>MRINHNIAALNTLNRLPSNNSASQKNMEKLSSGLRINRAGDDAAGLAISEKMRGQIRGLEMASKNSQDGISLIQTAEGALTETHAILQRVRELVVQAGNTGTQDKATDLQSIQDEISALTDEIDGISNRTEFNGKKLLDGTYKVDTATPANQKNLVFQIGANATQQISVNIEDMGADALGIKEADGSIAALHSVNDLDVTKFADNAADCADIGFDAQLKVVDEAINQVSSQRAKLGAVQNRLEHTINNLSASGENLTAAESRIRDVDMAKEMSEFTKNNILSQASQAMLAQANQQPQNVLQLLR[46x]

There are three parts to the flagellar structure: the trans-membrane basal body that functions as the motor, the connecting rod and hook, and the flagellar filament that acts like a helical propeller. Our current understanding of supercoiling in bacterial flagellar filaments, referred to as polymorphic switching, is based upon the notion that protofilaments within the flagellar filament can exist in two discrete states, that differ slightly in length. The “short” state results from a protofilament having a right-handed inclination (the R-state), while the “long” state results from a protofilament having a left-handed inclination (the L-state). To reconstruct filaments at high resolution, all protofilaments must be “locked” into the same state, either L- or R-type, producing straightened filaments that lead to non-motile bacteria.

While the three L-type mutants (E115G, S285P, and S17P) have a left-handed 11-start helix, the four R-type mutants (N226Y, A233V, H84R and A39VN133H) have a right-handed 11-start helix, and the designations L and R correspond to the hand of these 11-start helices. The L-type 11-start helices are tilted left by ~ 1.7° and the R-type 11-start helices are tilted right by ~ 3.9°. Strikingly, we found those sites are not necessarily conserved among different species or participate in unique inter-subunit interactions. These include three straight mutations outside of the D1 helices: S17P, S285P (both within D0) and the double mutant A39V/N133H (within the loop region). We also identified several straight mutations that are only involved in the 11-start interactions: S17P, H84R and A39V in the double mutants. We also detected two mutations, S17P and S285P, located in the middle of the small coiled-coil D0 domain. These two residues are not conserved in other species, and proline is not found at this position in any wildtype species. Therefore, mutation S17P or S285P in B. subtilis forces a local bend of ~ 30° in the helix axis, and this conformational change makes the D0 coiled-coil adopt an L-type form more easily. Here our high-resolution reconstructions expand our knowledge and we can now observe how mutations in D0 can cause a switching of the flagellar structure.>[2x]KSCC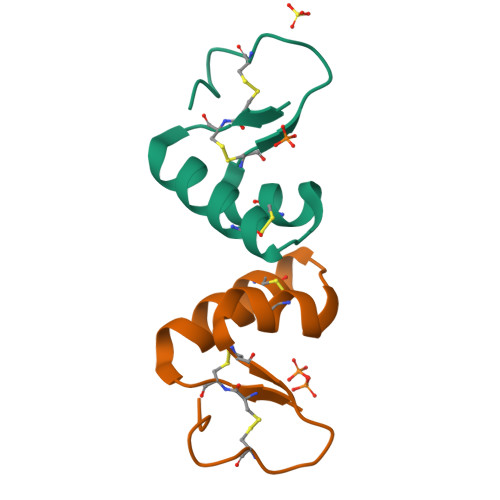PNTTGRNIYNACRLTGAPRPTCAKLSGCKIISGSTCPSDYPK> NNWEQQKKNIEDDLDRYKKRAEELRKEAEKARKEARKTEDPTEEAKKEWEKRCKELEERARKLEDEAKDRVNDLFDSNFFQVIYSGDNDEEEWKKEKDRAEKEIEEWFKRIKEKCEEIKKRLEQ;>SQDASDGLQRLHMLQISYFRDPYHVWYQGNASLGGHLTHVLEGPDTNTTIIQLQPLQEPESWARTQSGLQSYLLQFHGLVRLVHQERTLAFPLTIRCFLGCELPPEGSRAHVFFEVAVNGSSFVSFRPERALWQADTQVTSGVVTFTLQQLNAYNRTRYELREFLEDTCVQYVQKHISAENTKGSQTSRSYTS[2x]

A subset of PfEMP1 proteins bind to endothelial protein C receptor (EPCR), and their expression correlates with development of the symptoms of severe malaria. Structural studies revealed that PfEMP1 molecules present a helix-kinked-helix motif that forms the core of the EPCR-binding site. Binding of PfEMP1 prevents EPCR from binding to its natural ligand, protein C, thereby preventing PAR1-mediated endothelial signaling, most likely resulting in inflammation and endothelial dysfunction. In the absence of inhibitory antibodies against EPCR-binding PfEMP1 proteins, we instead used our knowledge of the structural features of the EPCR-binding site and grafted the core of this surface onto a three-helical bundle, which was redesigned through a Rosetta-based approach to produce a small synthetic protein that mimics the key features of the EPCR-binding surface.

The starting model for the designed immunogen contained residues N648 to K678 from the HB3var03 CIDRα1.4 domain inserted in between residues Gly70 and Asp103 of the three-helical bundle. We selected three sites in design 469 at which residues were predicted to be found at an appropriate distance to allow disulfide bond formation. These residues were replaced with cysteine to form three mutants, cys1, cys2, and cys3, each of which had a single disulfide bond. The cys2 variant was most effective, retaining α-helicity at up to 70°C in circular dichroism measurements and interacting with EPCR with a slow off-rate, reminiscent of the CIDRα1-EPCR interaction. As determined by surface plasmon resonance, the cys2 variant bound to EPCR with an affinity of 26 nM, which compares well with 220 nM for the D576A K642A mutant of this domain, which shares the same number of EPCR-binding residues as cys2. We next determined the crystal structure of the synthetic binder in complex with EPCR. Crystals formed and a complete data set was collected to 3.11 Å resolution. Surprisingly, a cycle of refinement and model building revealed the presence of a single copy of the synthetic binder, with the asymmetric unit containing a complex of EPCR bound to a synthetic binder, together with a second, unliganded, copy of EPCR. A structural alignment revealed the EPCR-binding site to adopt an extremely similar conformation to that predicted, with the residues of the helix-kinked-helix motif of the synthetic binder (N72-W93) overlaying with the design with a RMSD of 1.19 Å. The structure also revealed that the synthetic binder bound to EPCR with the same binding mode as the HB3var03 CIDRα1 domain. Indeed, aligning these two complexes on the EPCR molecule showed the residues of the helix-kinked-helix of the synthetic binder (N72 to W93) to overlay with the corresponding residues of the HB3var03 CIDRα1.4 domain (N648-W669) with an RMSD of 0.77 Å.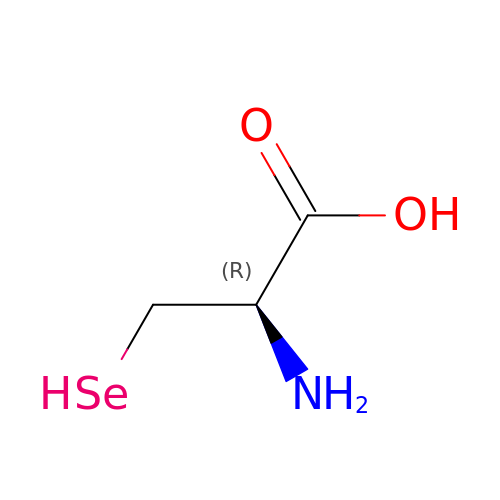SELENOCYSTEINE | C3 H7 N O2 Se | ZKZBPNGNEQAJSX-REOHCLBHSA-N> GGFVAHVESTCLLDDAGTPKDFTYCISFNKDLLTCWDPEENKMAPCNSLANVLSQHLNQKDTLMQRLNGLQNCATHTQPFWGSLTNRTRPPSVQVAKTTPFNTREPVMLACYVWGFYPAEVTITWRKNGKLVM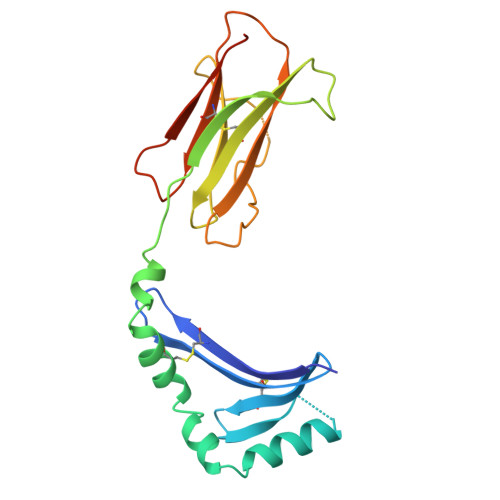HSSAHKTAQPNGDWTYQTLSHLALTPSYGDTYTCVVEHIGAPEPILRDWTPGLSPMQTLK Here, the ligand‐free crystal structure of UMG‐SP2, a metagenome‐derived urethanase with depolymerization activities, at 2.59 Å resolution, as well as its (co‐)structures bound to a suicide hydrolase inhibitor and a short‐chain carbamate substrate at 2.16 and 2.40 Å resolutions, respectively, is reported. UMG‐SP2 belongs to the amidase signature protein superfamily (AS family), which is characterized by a highly conserved GGSS(S/G)GS motif and can be found in bacteria, archaea, and eukaryotes. SP2 shares the domain architecture of amidases, with an α/β‐fold containing 12 prominent α‐helices, 12 β‐strands, and five larger loops. Structural analysis and molecular dynamics simulations reveal that the flexible loop L3 consisting of residues 219–226 is crucial for regulating the hydrolytic activity of UMG‐SP2.

In addition, a SP2 variant with the catalytic triad serine mutated to alanine (S190A) was created and used to solve the complex structure (SP2S190A, 2.40 Å resolution) with the model substrate 4‐hydroxybutyl (4‐(4‐aminobenzyl)phenyl) carbamate (BBC) containing a urethane bond. The structures of SP2S190A and SP2 were solved by MR based on the refined structure of SP2PMS omitting the covalently modified S190. Likewise, when bound to the primary active site cavity of the inactive mutant SP2S190A, the phenyl moiety of the substrate BBC adopts a similar pose as PMS, with the scissile urethane bond in the vicinity of A190 (left inset). The aliphatic 4‐hydroxybutyl moiety of BBC crosses the oxyanion hole and enters a secondary cavity separate from the active site. The hydrophobic residues L140 and I187 bind to the 4‐hydroxy butyl moiety of the BBC ligand and form the secondary cavity of the active site, which partially accommodates BBC. Only one region near the active site of the substrate‐bound SP2S190A, belonging to the loop L3 (residues 219–226, corresponding to the loop L3 also found in UMG‐SP1), has a different conformation than the other structures and the computational model SP2AF2. Upon binding of BBC, K224, and concomitantly the flanking residues A223 and A225 perform a backbone flip that leads to a release of the active site steric blockage and the K224 side chain now points into the solvent as seen in the SP2S190A structure complexed with BBC (right insert). Interestingly, we discovered a second substrate binding site that is only found in the second molecule of the asymmetric unit of the BBC‐bound SP2S190A complex structure. R325, on the other hand, can directly interact with substrate in the secondary site, through the amphipathic part of the side chain or hydrogen bonds, since the guanidine group of R325 is within 4 Å of BBC's carbamate group, both of which are abrogated by replacing R325 with the smaller alanine.

>NLYFQGAGAGAGAGAMSELSAIETAAAIAGGSMTALEACDAAIARIEQRDGPINAVVVRDFDRARDAAKAADAEIAAAVRKPLLGVPMTIKESFDIAGLPTSWGFAEHADHIATADSLVVSRLKAAGAVFLGKSNIPVGLADWQSVNPNYGRTNNPHDHSRSAGGSSGGAAAALAAGMVPLEYGSDIGGAIRVPAHFCGVWGLKTTFDAVSLEGHYFPRTDSAKADLSVVGPMARTPADLALALDITSKVPLPQSRIANLSGLRILLLTAHPETVADSATISAVERAAAACEASGATVATSSPDLPDLSALVADYTRMLLVVLARGLAPEGTEPVSLNAWYAMLDDQARMMRAFDRLFESFDAIFCPVLGTTAFAHSDEPDWAKRSLSIDGGIAPFAAQLGWISMATYGGMPALSMPLGADGNGLPINLQIITRNWSDHDAIRIGALVAEALDR[2x]> MGVEKVPKYDIPVKKVEYVFIELDKMKPHEQLVQRELEDFIESVTGSGIFWKPMLLAKIPGTDEYLIVDGHHRWAGLQKLGAKRAPSVILDYFDEGVKVYTWYPAFKGDVNKVIERLKAEGLEVIEDEKAEEKAEKGEIAFALIGEKSFAIPGGLEEQKKVSKVLDEMDQAKEIELVYYGLKEDAKADMEKGEIDYVF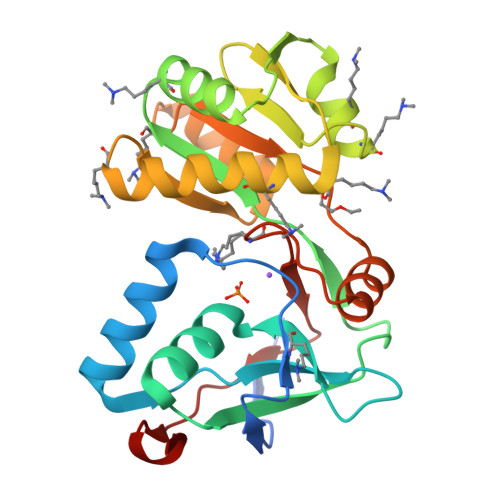IRKAPTKEEVMELVKRGEVFSPKTTRHVLPFIPDKIDVKLEDLF> GSHMATIRNLKIKTSTCKRIVK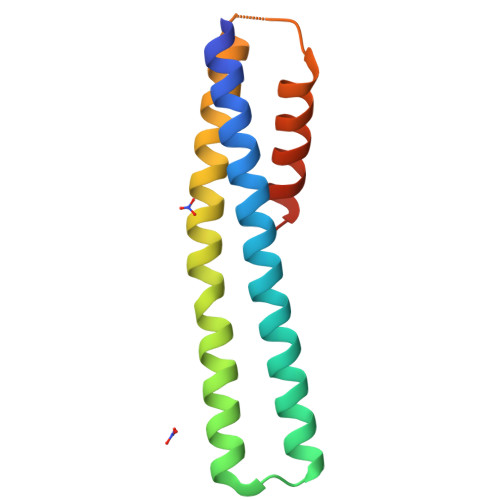ELHSYEKEVEREAAKTADMKDKGADPYDLKQQENVLGESRMMIPDCHKRLESALADLKSTLAELEETDEKEGPEIEDAKKTVADVEKQFPTEDA> MERSTRE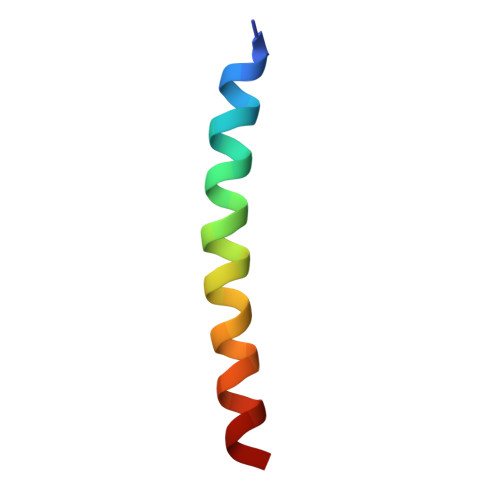LCLNFTVVLITVILIWLLVRSYQY> GSMDSDLKAKVESCARTADTFTRLYYASVDNRRQQIGRLYLDNATLSWNGNGAIGRQMIESYFQELPSSNHQLNTLDAQPIVDQAVSNQLAYLIMASGSVKFADQQLRKFQQTF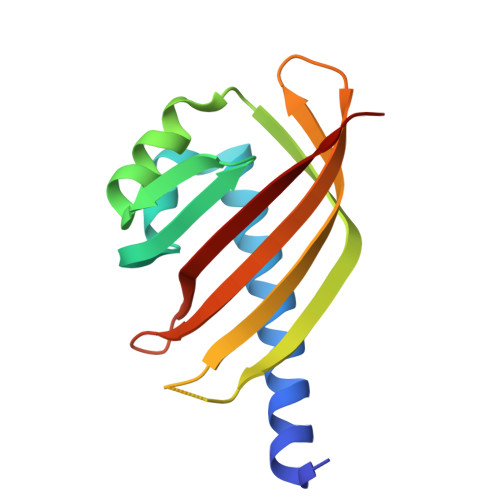IVTAENDKWKVVSDCYRMQEV Human glycolipid transfer protein (hsGLTP) forms the prototypical GLTP fold and is characterized by a broad transfer selectivity for glycosphingolipids (GSLs). In human GLTP, a glycolipid headgroup recognition centre located on the protein surface enables selective binding of the GSL head and ceramide amide groups via multiple specific interactions. Encapsulation of lipid chains within the hydrophobic pocket involves a cleft-like gating mechanism that results in two glycolipid-binding modes. To elucidate the structural dynamics of the GLTP–GSL dimer and associated adaptations, we comparatively analyzed nine novel crystal structures of wild-type GLTP (wtGLTP) and the sulfatide-specific mutants D48V and A47D/D48V complexed with N-lauroyl-containing monosulfatide (N-lauroyl-3-O-sulfo-galactosylceramide; hereafter referred to as 12:0 monoSF) and disulfatide (N-lauroyl-3,6-di-O-sulfo-galactosylceramide; hereafter referred to as 12:0 diSF) in different crystal forms and compared them with previously studied GLTP–24:1 monoSF complexes.

The GLTP mutation D48V near the ‘portal entrance’ of the glycolipid binding site has recently been shown to enhance selectivity for sulfatides (SFs) containing a long acyl chain. Compared with wtGLTP dimers, all dimers of D48V mutant are locked. Compared with the wild-type protein, some interfacial regions in the D48V dimer contain noticeably expanded intermolecular contacts. The first region involves the α2–α2′ hydrophobic core formed by residues Pro44, Ala47 and Val48 with their counterparts, as was originally found in the D48V mutant complexed with 24:1 monoSF in the sphingosine-in binding mode. Since the same core becomes the major protein–protein′ contact in the D48V dimer complexed with 12:0 monoSF, we were surprised to discover the sphingosine chain projecting outwards and entering the partner hydrophobic pocket in the sphingosine-out binding mode. In turn, the lipid–lipid′ and the lipid–protein′ interactions become weaker in the dimer of the D48V mutant as indicated by the reduced number of interatomic close contacts, which are reminiscent of those encountered in the sphingosine-in binding mode of 24:1 monoSF complexed with the same mutant. Only ‘closed’ conformations characterized by a very narrow range of θ angles (62.6–65.5°) are observed in different complexes/crystals. The extra monomer–monomer interactions arising in the mutant and described in detail in the next section stabilize the closed conformation of D48V–SF dimers, which we therefore refer to as a ‘locked dimer’. The diminished monomer–monomer′ contact areas of the D48V–SF dimers imply reduced stabilities, which decrease despite the expanded protein–protein′ contacts (1300–1310 versus 1020–1090 Å2 in wtGLTP), again emphasizing the importance of the bound ligand for GLTP dimerization.

> MALLAEHLLKPLPADKQIETGPFLEAVSHLPPFFDCLGSPVFTPIKAVISGNITKIKAVYDTNPAKFRTLQNILEVEKEMYGAEWPKVGATLALMWLKRGLRFIQVFLQSICDGERDENHPNLIRVNATKAYEMALKKYHGWIVQKIFQAALYAAPYKSDFLKALSKGQNVTEEECLEKIRLFLVNYTATIDVIYEMYTQMNAELNYKV> XRMKQIEDKIEEIESKQ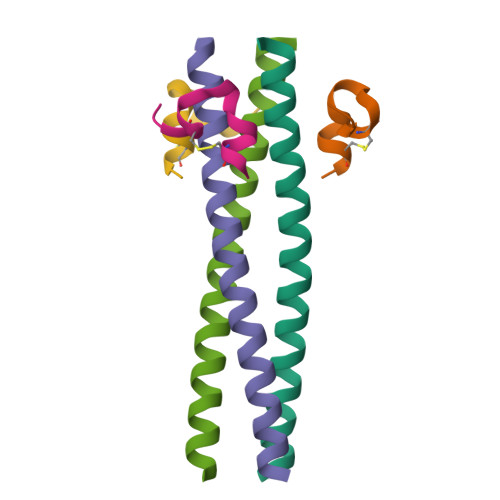KKIENEIARIKKLLQLTVWGIKQLQARILX;> XKGHPCDYPEWQWLCELX>[8x]MAGSNDVAKVMKTLDGMREGLIQTAVELGSIEAPTGREGAAGDYVYEWMARNGFGPERVGVFDDRFNVVGRLRGTGGGASLSFNSHLDTIMAREDTARFADANDRIYHEAWHEEGRIYGYSVVNCKGPMACWLIAAKALKEAGAALKGDVVLTAVCGEIDCEPVDEFQGHDYLAEDIGARYAISHGAISDYALVAEATNFKPAWVEA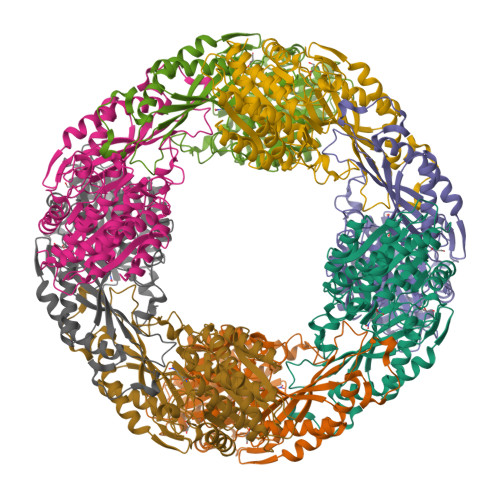GKVFLKVTVFAGPSRYTPYVPRPVAALDSPNAIVRMAKLVEALEEWADNYEKRYTREYGGGTVVPKVAIGAIRGGVPYKIYAFPELCSIYMDIRLNPDTNPLVVQREVEAVVSKLGLKAEVKPFLFRRGYEAQGIEPLQNALEVAHREVVGRPTERPGSPECSMWRDTNPYNELGIPSLTYGCGGGAGGGNTYFLVDDMLKAAKVYAMTAMDLCNRTP> DRHHHHHHKLSRAHDNQPGTIRSDHYTCVGCVLVVSVI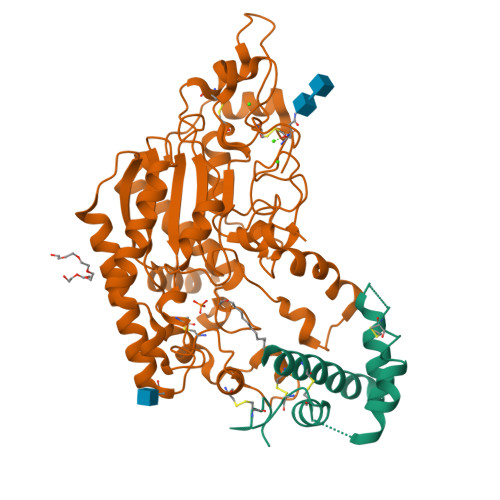EQLAQVHNSTVQASMERLCSYLPEEWVLKTACYMMVHVFGADIIKLFDKDVNADVVCHTLEFCKQEPGQPLCHLYPLPKESWKFTLEKARHIVKQSPIMKYTR;> SGAGICSLPFLAKICQKIKLAIKNSVPIKDVDSDKYSIFPTLRGYHWRGRDCNDSDKTVYPGRRPDNWDAHRDSNCNGIWGVDPKDGIPYEKKFCEGSQPRGIILLGDAAGAHFHIPPEWLTVSQMSVNSFLNLPTAVTNELDWPQLSGTTGFLDSASKIKENSIYLRLRKRNRCNHRDYQNISKNGASSRNVKSLIESLSRNQLLDHPAIVIYAMIGNDVCNGRKTDPVSAMTTPEQLYANVLKMLEALNSHLPTGSHVILYGLAHGAFLWDTLHSRYHPLGQLNKDVTYTQLYSFLGCLQVSPCPGWMSANETLRALTSERAQQLSETLRKIAASKKFTNFNLFYLDFAFQEVVEEWQKMGGQPWELIEAVDGFHPNEVALLLFADQLWEKVQRQWPDVLGKENPFNPQIEEVFGDQGGH> SNAMSFIAIIPARYASTRLPGKPLADIAGKPMVVHVMERALASGADRVIVATDHPDVVKAVEAAGGEVCLTRA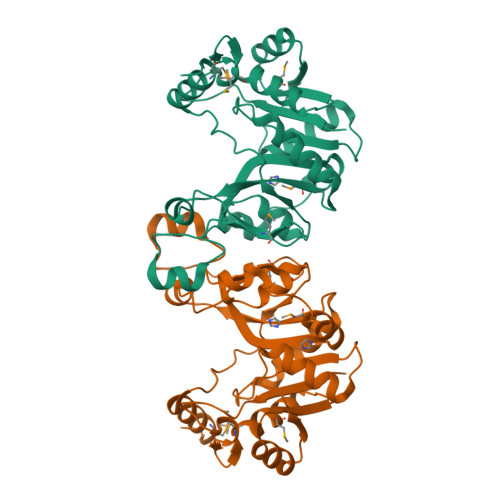DHQSGTERLAEVIEHYGFADDDIIVNVQGDEPLVPPVIIRQVADNLAACSAGMATLAVPIASSEEAFNPNAVKVVMDAQGYALYFSRATIPWERERFAQSKETIGDCFLRHIGIYAYRAGFIRRYVNWAPSQLEQIELLEQLRVLWYGEKIHVAVAKAVPAVGVDTQSDLDRVRAIMLNQ Bromodomains (BRDs) are protein interaction modules that specifically recognize ε-N-lysine acetylation motifs, a key event in the reading process of epigenetic marks. The 61 BRDs in the human genome cluster into eight families based on structure/sequence similarity. Despite large sequence variations, all BRD modules share a conserved fold that comprises a left-handed bundle of four α helices (αZ, αA, αB, αC), linked by loop regions of variable length (ZA and BC loops), which line the Kac binding site and determine binding specificity. The four helices form a deep cavity that is extended by the two loop regions (ZA and BC loops), creating a largely hydrophobic Kac binding pocket.

The second BET BRDs bound to tetra-acetyl H4 peptides with about 10-fold weaker affinities, suggesting that the first BRD in BET proteins recognizes the H4 tail. In contrast, the second BRDs of BET BRDs bound either weakly (BRD2), not at all (BRD3), or promiscuously (BRD4) to histone sequences and their variants present in this array. For instance, recurrent t(15;19) chromosomal translocations that result in a fusion protein that comprises both BRD4 or BRD3 and the NUT (nuclear protein in testis) lead to an aggressive form of human squamous carcinoma (French, 2010a; French et al., 2001).

>[4x]SMGKLSEHLRYCDSILREMLSKKHAAYAWPFYKPVDAEALELHDYHDIIKHPMDLSTVKRKMDGREYPDAQGFAADVRLMFSNCYKYNPPDHEVVAMARKLQDVFEMRFAKMP> GPLGSEVVRCICEVQEENDFMIQCEECQSWQHGVCMGLLE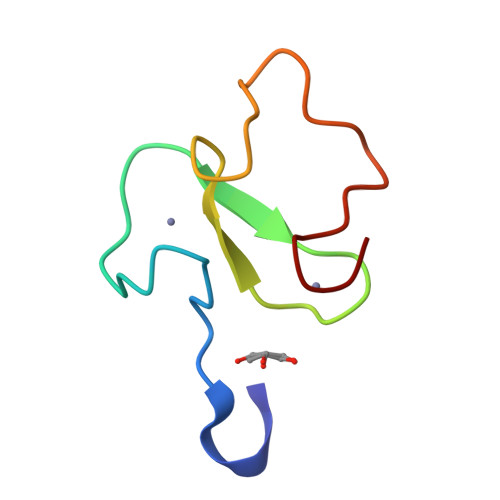ENVPEKYTCYVCQ>[4x]SNAMGTKNIGKGLTFEDILLVPNYSEVLPREVSLETKLTKNVSLKIP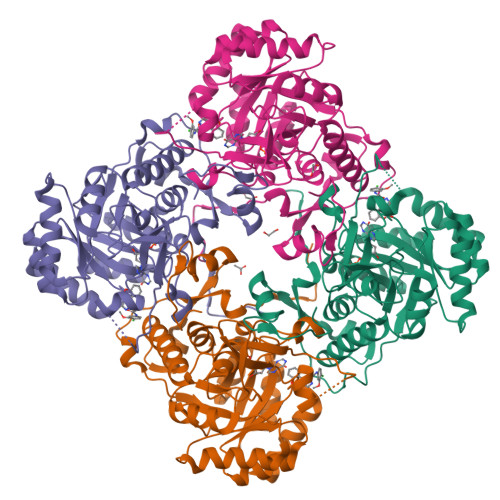LISSAMDTVTEHLMAVGMARLGGIGIIHKNMDMESQVNEVLKVKNSGGLRVGAAIGVNEIERAKLLVEAGVDVIVLDSAHGHSLNIIRTLKEIKSKMNIDVIVGNVVTEEATKELIENGADGIKVGIGPGSICTTRIVAGVGVPQITAIEKCSSVASKFGIPIIADGGIRYSGDIGKALAVGASSVMIGSILAGTEESPGEKELIGDTVYKYYRGMGSVGAMKSGSGDRYFQEKRPENKMVPEGIEGRVKYKGEMEGVVYQLVGGLRSCMGYLGSASIEELWKKSSYVEITTSGLRESHVHDVEIVKEVMNYSK>[2x]MASKKPDKTYEEMVKEVERLKLENKTLK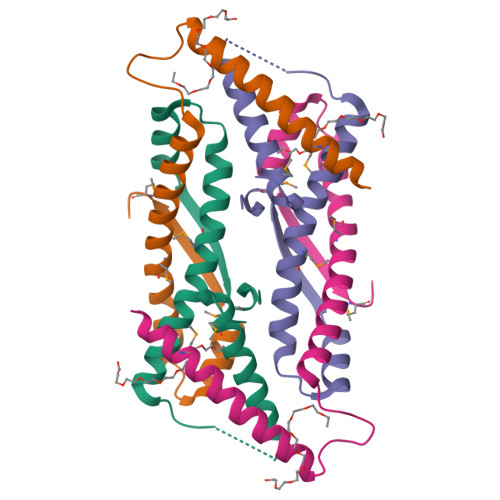QKVKSSGAVSSDDSILTAAKRESIIVSSSRALGAVAMRKIEAKVRSRAAKAVTEQELTSLLQSLTLRVDVSMEELEHHHHHH>[8x]MGSIGEPNRLLCWSIYVTKKPDQSEEDHHNHVSKVNAPMFIP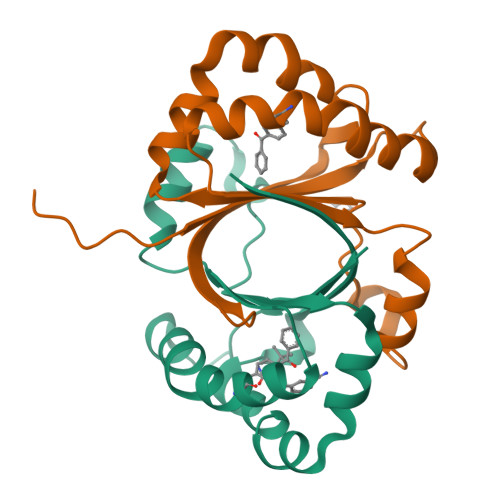FLKKYGIVRYTVKHNDAYSKPKQAALMAGQPEENVLAYDTVFEIIVKDIESIQTMQKDEEFLRTTIPDHFNFADMTRSKGSLTWIEEFTFALEHHHHHH>ADIIGGLAYTMGGRCSVGFAATNASGQPGFVTAGHCGSVGTQVSIGNGRGVFERSVFPGNDAAFVRGTSNFTLTNLVSRYNSGGYATVSGSSTAPIGSQVCRSGSTTGWYCGTIQARNQTVSYPQGTVHSLTRTSVCAEPGDSGGSFISGTQAQGVTSGGSGN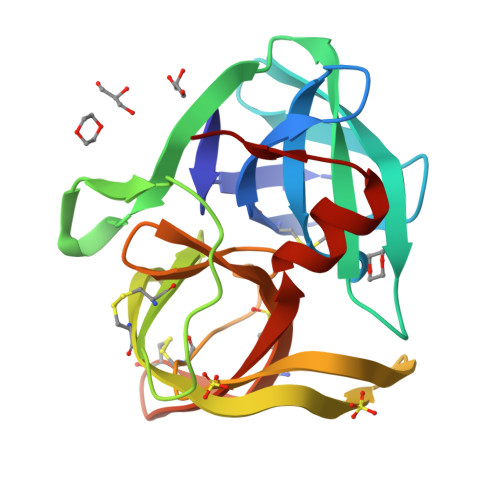CRTGGTTFYQEVNPMLNSWNLRLRT[2x]>[2x]MGSDKIHHHHHHMIEYRIEEAVAKYREFYEFKPVRESAGIEDVKSAIEHTNLKPFATPDDIKKLCLEARENRFHG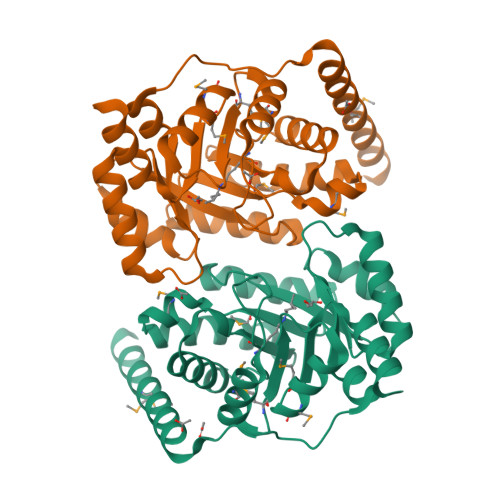VCVNPCYVKLAREELEGTDVKVVTVVGFPLGANETRTKAHEAIFAVESGADEIDMVINVGMLKAKEWEYVYEDIRSVVESVKGKVVKVIIETCYLDTEEKIAACVISKLAGAHFVKTSTGFGTGGATAEDVHLMKWIVGDEMGVKASGGIRTFEDAVKMIMYGADRIGTSSGVKIVQGGEERYGG>MAGDTTITVVGNLTADPELRFTPSGAAVANFTVASTPRMFDRQSGEWKDGEALFLRCNIWREAAENVAESLTRGSRVIVTGRLKQRSFETREGEKRTVVEVEVDEIGPSLRYATAKVNKASRSGGGGGGFGSGGGGSRQSEPKDDPWGSAPASGSFSGAD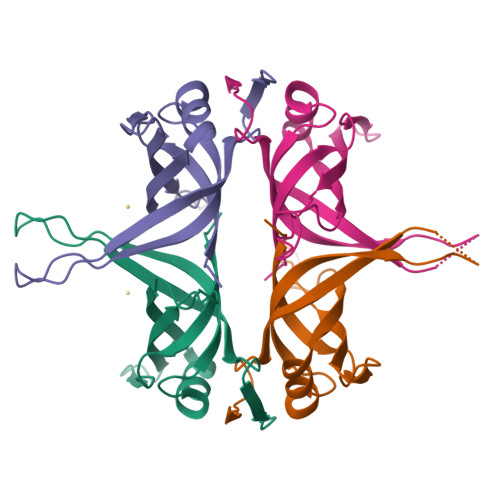DEPPF[2x]5-[(Z)-2-fluoro-2-(4-hydroxyphenyl)ethenyl]benzene-1,3-diol 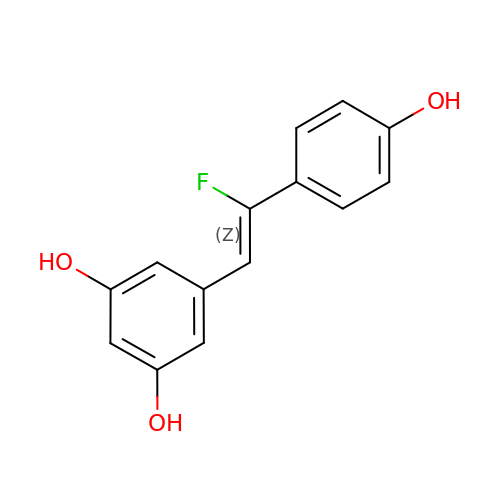| C14 H11 F O3 | PNBPFKSSWYNPPD-AUWJEWJLSA-N> MGCVSSKSTTVLSPQTSFNEASRTSFRALPGPSQRQLEVYDQCLIGAARWPDDSSKSNTPENRAYCQSMYNSIRSAGDEISRGGITSFEELWGRATEWRLSKLQRGEPLYSAFASERTSDTDAVTPLVKPYKSVLARVVDHEDAHDEIMQDNLFGDLNVKVYRQTAYLHGNVIPLNTFRVATDTEYLRDRVAHLRTELGAKALKQHLQRYNPDRIDHTNASYLPIIKDHLNDLYRQAISSDLSQAELISLIARTHWWAASAMPDQRGSAAKAEFAARAIASAHGIELPPFR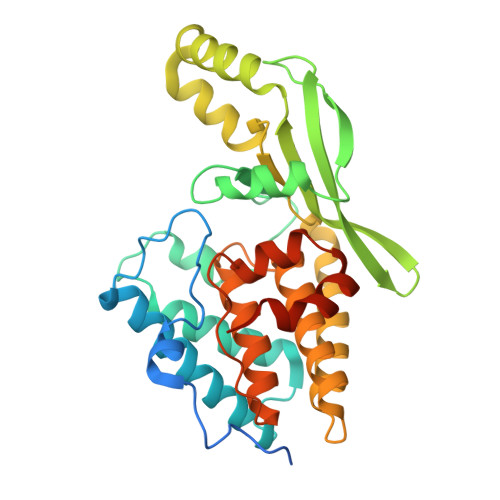NGNVSDIEAMLSGEEEFVEKYRSLLDSDCFGTGHHHHHH>MGWHHHHHHENLYFQGASMKLVIARVKSPKVKRLSEEDIEKIKSALKSTNKAVVTIKDENGEEIEVEVRLLTLEEALKYINDLPISNDAKKLMSNNIHKALEPGRTVVFGPEGCEERDKNRGIIKTFSTDVKLDETYFFFRVEAE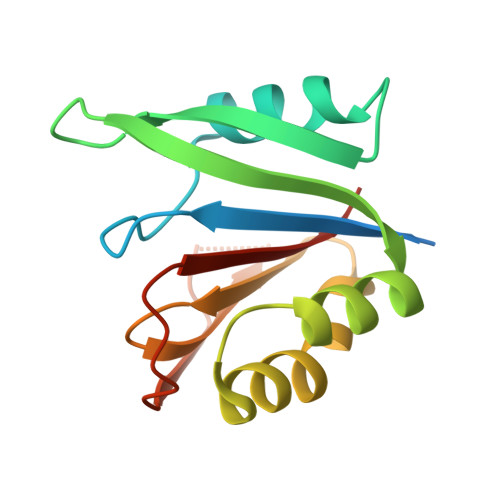Q[4x]> GHMVPVVCEVVSEAIVHAAQKLKEYLGFEYPPSKLCPAANTLNEIFLIHFITFCQEKGVDEWLTTTKMTKHQAFLFGADWIWTFWGS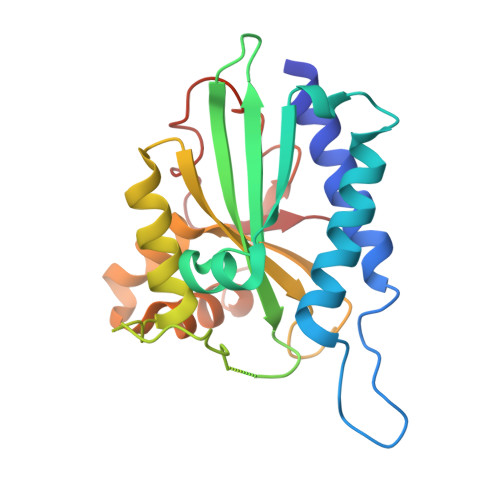DKQIKLQLAVQTLQMSSPPPVESKPCDLSNPESRVEESSWKKSRFDKLEEFCNLIGEDCLGLFIIFGMPGKPKDIRGVVLDSVKSQMVRSHLPGGKAVAQFVLETEDCVFIKELLRNCLSKKDGLREVGKVYISIL> SSPTSLTNVTIFSPPSDYIVPRTLYPRNEQLPNGDLLATWENYSPEPPAVYFPIYRSKDHGKTWNEISRVHDTVNGYGLRYQPFLYSLPERVGSFKKGTLLLAGSSIPTDLSSTDIVLYASQDDGMTWDFVSHIAAGGEARPNNGLTPVWEPFLLANKGKLICYYSDQRDNATYGQTMVHQVTNDLKNWGPVVEDVTYPTYTDRPGMPVVTKLPNG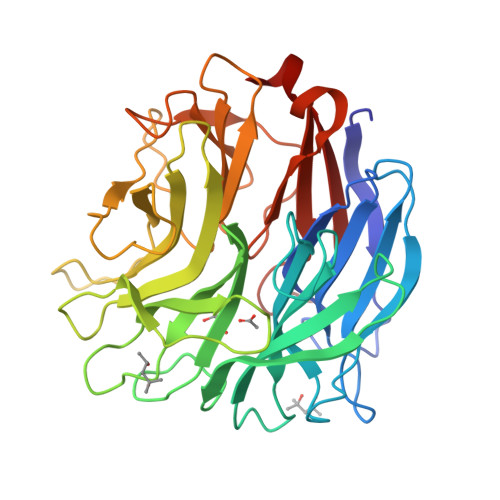QYFYVYEYGSFFGTETYSFPLYYRLSSDPENIASAPGQRLVVSSGTQPTSSPYAVWTPYGGENGTIIVSSGTQGTLFINKALGEGEWTEIPCPEEHGYTRALRVLSEDGGRYLVVNSAGVLLGENNRVSVSVMDLKEVL(2~{S})-2-[[(2~{S})-3-[4-(5-ethanoyl-2-fluoranyl-phenyl)phenyl]-2-(3-oxidanylidene-1~{H}-isoindol-2-yl)propanoyl]amino]propanoic acid | C28 H25 F N2 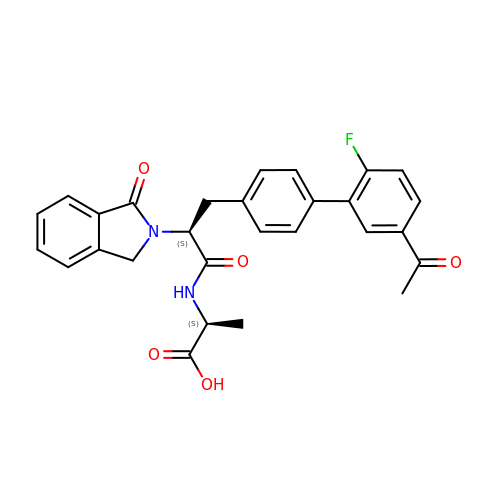O5 | TXGHAFIFHKHLOM-LMKMVOKYSA-N> LPYF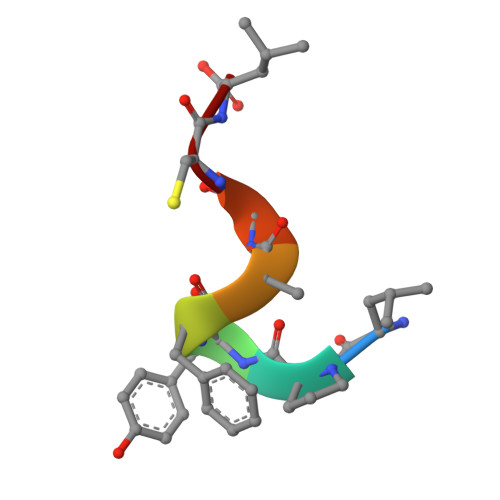AGCL> AIGEFMVSLPRMVYPQPKVLTPCRKDVLVVTPWLAPIVWEGTFNIDILNEQFRLQNTTIGLTVFAIKKYVAFLKLFLETAEKHFMVGHRVHYYVFTDQPAAVPRVTLGTGRQLSVLEVRAYKRWQDVSMRRMEMISDFCERRFLSEVDYLVCVDVDMEFRDHVGVEILTPLFGTLHPSFYGSSREAFTYERRPQSQAYIPKDEGDFY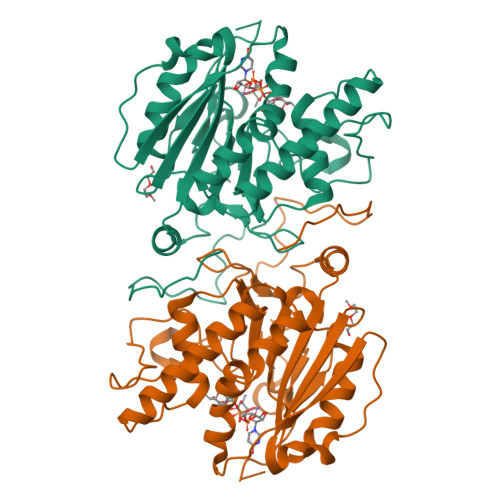YMGGFFGGSVQEVQRLTRACHQAMMVDQANGIEAVWHDESHLNKYLLRHKPTKVLSPEYLWDQQLLGWPAVLRKLRFTAVPKNHQAVRNPE> GLIVDTRDVEERVHVMRKTKLAPTVAHGVFNPEFGPAALSNKDPRLNEGVVLDEVIFSKHKGDTKMSAEDKALFRRCAADYASRLHSVLGTANAPLSIYEAIKGVDGLDAMEPDTAPGLPWALQGKRRGALIDFENGTVGPEVEAALKLMEKREYKFACQTFLKDEIRSMEKVRAGKTRIVDVLP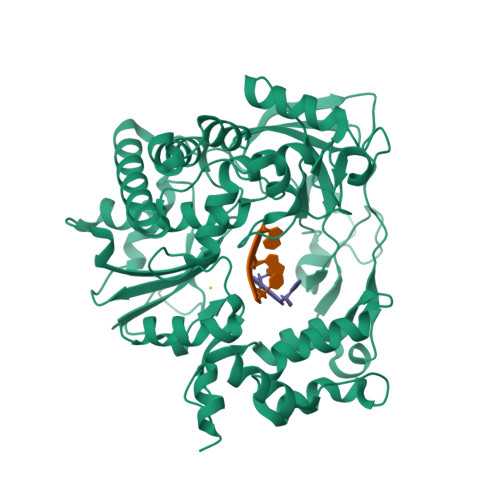VEHILYTRMMIGRFCAQMHSNNGPQIGSAVGCNPDVDWQRFGTHFAQYRNVWDVDYSAFDANHCSDAMNIMFEEVFRTEFGFHPNAEWILKTLVNTEHAYENKRITVEGGMPSGCSATSIINTILNNIYVLYALRRHYEGVELDTYTMISYGDDIVVASDYDLDFEALKPHFKSLGQTITPADKSDKGFVLGHSITDVTFLKRHFHMDYGTGFYKPVMASKTLEAILSFARRGTIQEKLISVAGLAVHSGPDEYRRLFEPFQGLFEIPSYRSLYLRWVNAVCGDAAALAHH6-(2-{3-[3-(dimethylamino)propyl]-5-(trifluoromethyl)phenyl}ethyl)-4-methylpyridin-2-amine | C20 H26 F3 N3 | 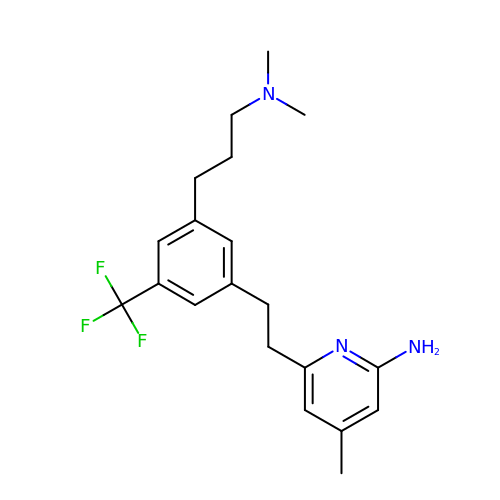CTKGSJUPWJLHAK-UHFFFAOYSA-N> GSHMESGNAQDGDLEDADADDHSFWCHSQLEVDGSQHLLTCAFNDSDINTANLEFQICGALLRVKCLTLNKLQDIYFIKTSEFLLIGSSNICVKLGQKNLTCKNMAINTIVKAEAPSDLKVVYRKEANDFLVTFNAPHLKKKYLKKVKHDVAYRPARGESNWTHVSLFHTRTTIPQRKLRP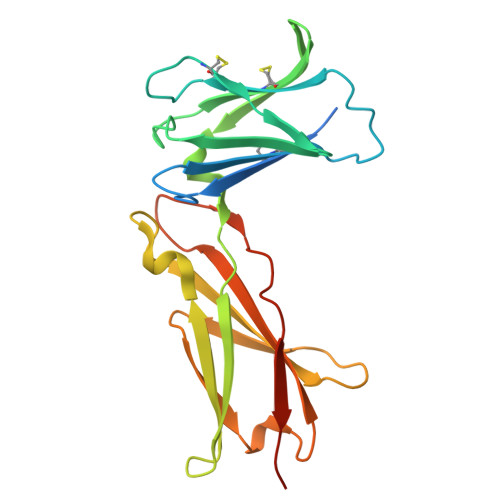KAMYEIKVRSIPHNDYFKGFWSEWSPSSTFETPEPKNQGGWD> MELTLWTYEGPPHIGAMRIATSMKGLHYVLHAPQGDTYADLLFTMIERRGSRPPVTYTTFQARDLGGDTAELVKGHIFEAVERFKPEALLVGESCTAELIQDQPGSLAKGMGLNIPIVSLELPAYSKKENWGASETFYQLIRGLLKEISEDSSNNAKQSWQEEGRRPRVNLLGPSLLGFRCRDDVLEIQKILGENGIDINVIAPLGASPSDLMRLPKADANVCLYPEIAESTCLWLERNFKTPFTKVVPIGVKATQDFLEELYELLGMEVSNSISNSDQSKLPWYSKSVDSNYLTGKRVFIFGDGTHVLAAARIANEELGFEVVGIGTYSREMARKVRAAATELGLEALITNDYLEVEESIKECAPELVLGTQMERHSAKRLGIPCAVISTPMHVQDVPARYSPQMGWEGANVIFDDWVHPLMMGLEEHLIGMFRHDFEFTDGHQSHLGHLGGHASETKTSSKGINQSPNNHSPAGESIHWTSEGESELAKIPFFVRGKVRRNTEK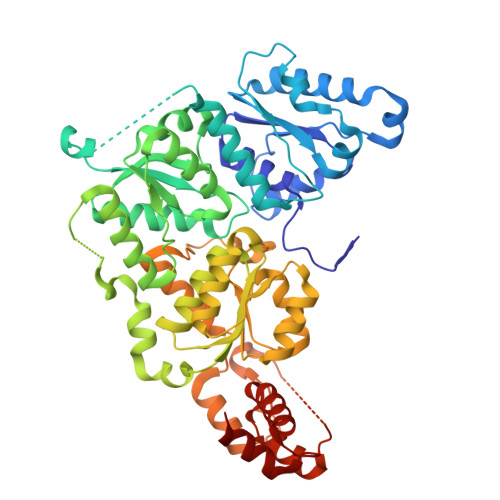YARQAGCREIDGETLLDAKAHFGA> MGSSHHHHHHSQSGSGMTTLKLDTLSDRIKAHKNALVHIVKPPVCTERAQHYTEMYQQHLDKPIPVRRALALAHHLANRTIWIKHDELIIGNQASEVRAAPIFPEYTVSWIEKEIDDLADRPGAGFAVSAANARVLHEVCPWWRGQTVQDRCYGMFTDEQKGLLATGIIKAEGNMTSGDAHLAVNFPLLLEKGLDGLREEVAERRSRINLTVLEDLHGEQFLKAIDIVLVAVSEHIERFAALAREMAATETRESRRDELLAMAENCDLIAHQPPQTFWQALQLCYFIQLILQIESNGHSVSFGRMDQYLYPYYRRDVELNQTLDREHAIEMLHSCWLKLLEVNKIRSGSHSKASAGSPLYQNVTIGGQNLVDGQPMDAVNPLSYAILESCGRLRSTQPNLSVRYHAGMSNDFLDACVQVIRCGFGMPAFNNDEIVIPEFIKLGIEPQDAYDYAAIGCIETAVGGKWGYRCTGMSFINFARVMLAALEGGHDATSGKVFLPQEKALSAGNFNNFDEVMDAWDTQIRYYTRKSIEIEYVVDTMLEENVHDILCSALVDDCIERAKSIKQGGAKYDWVSGLQVGIA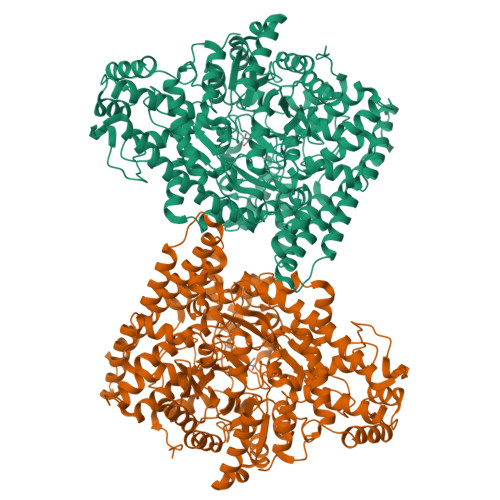NLGNSLAAVKKLVFEQGAIGQQQLAAALADDFDGLTHEQLRQRLINGAPKYGNDDDTVDTLLARAYQTYIDELKQYHNPRYGRGPVGGNYYAGTSSISANVPFGAQTMATPDGRKAHTPLAEGASPASGTDHLGPTAVIGSVGKLPTAAILGGVLLNQKLNPATLENESDKQKLMILLRTFFEVHKGWHIQYNIVSRETLLDAKKHPDQYRDLVVRVAGYSAFFTALSPDAQDDIIARTEHML>[2x]GSHMTKALYDRDGAAIGNLQKLRFFPLAISGGRGARLIEENGRELIDLSGAWGAASLGYGHPAIVAAVSAAAANPAGATILSASNAPAVTLAERLLASF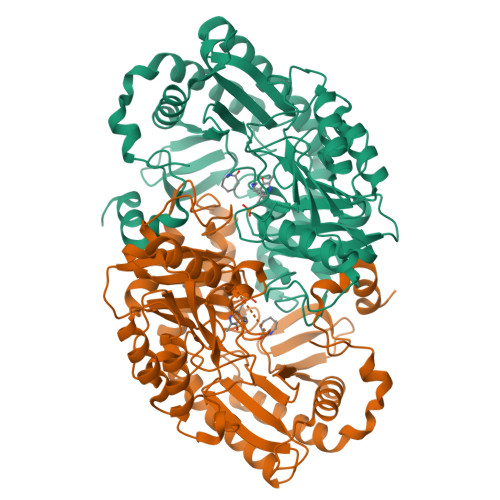PGEGTHKIWFGHSGSDANEAAYRAIVKATGRSGVIAFAGAYHGCTVGSMAFSGHSVQADAAKADGLILLPYPDPYRPYRNDPTGDAILTLLTEKLAAVPAGSIGAAFIEPIQSDGGLIVPPDGFLRKFADICRAHGILVVCDEVKVGLARSGRLHCFEHEGFVPDILVLGKGLGGGLPLSAVIAPAEILDCASAFAMQTLHGNPISAAAGLAVLETIDRDDLPAMAERKGRLLRDGLSELAKRHPLIGDIRGRGLACGMELVCDRQSREPARAETAKLIYRAYQLGLVVYYVGMNGNVLEFTPPLTITETDIHKALDLLDRAFSELSAVSNEEIAQFAGW>[2x]MSKQPMTPFEAIGGEQCIEILVDTFYSYVSKHPDLSPIFPDDLTETARKQKQFLTQYLGGPN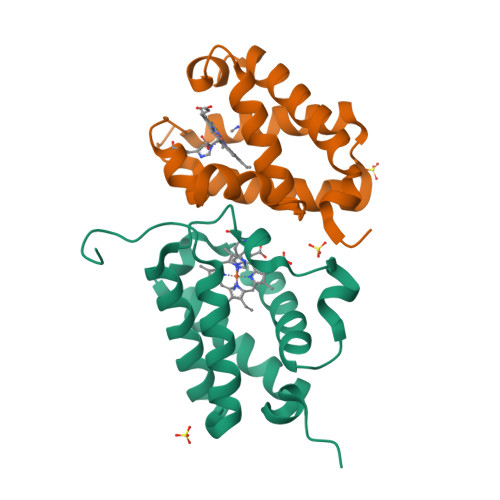LYTEEHGHPMLRARHLPFEITPKRAEAWLSCMEQAMDDTGVHGHIREFVFERLALTAQHMVNTPNETGEI> MNILQEPIDFLKKEELKNIDLSQMSKKERYKIWKRIPKCELHCHLDLCFSADFFVSCIRKYNLQPNLSDEEVLDYYLFAKGGKSLGEFVEKAIKVADIFHDYE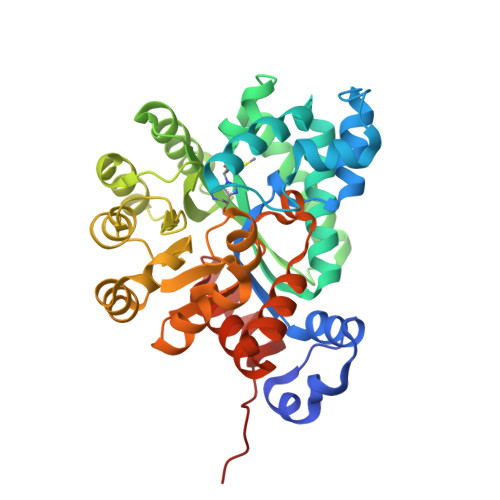VIEDLAKHAVFNKYKEGVVLMEFRYSPTFVAFKYNLDIELIHQAIVKGIKEVVELLDHKIHVALMCIGTGHEAANIKASADFCLKHKADFVGFDHGGHEVDLKEYKEIFDYVRESGVPLSVHAGEDVTLPNLNTLYSAIQVLKVERIGHGIRVAESQELIDMVKEKNILLEVCPISNVLLKNAKSMDTHPIRQLYDAGVKVSVNSDDPGMFLTNINDDYEELYTHLNFTLEDFMKMNEWALEKSFMDSNIKDKIKNLYFKGEFEAYV> SQSNRELVVDFLSYKLSQKGYSWSQMAAVKQALREAGDEFELRYRRAFSDLTSQLHITPGTAYQSFEQVVNELFRDGVNWGRIVAFFSFGGALCVESVDKEMQVLVSRIAAWMATYLNDHLE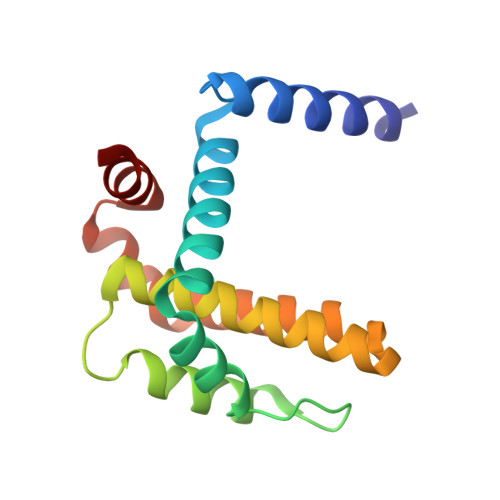PWIQENGGWDTFVELYGN> GSHMELTTTAARPGLRHRMQQLIYGFFTAQTLHVAVRLRIPDLLADGARDVGDLASATGADAPSLRRLLRALVFLEVLDEPAPGTFALTEQGEVLRADVTGSMRELVLLLSGPESWAAWGQLEHSVRTGEVAWEHVHGRSCFDHLMADPQRQAAFNAAMAEGSRAFVPTLLSAYDFGDLRTVVDVGGGSGALLAGVLAAHPHLRGTVFDTPDGVADAARTVAEQGVA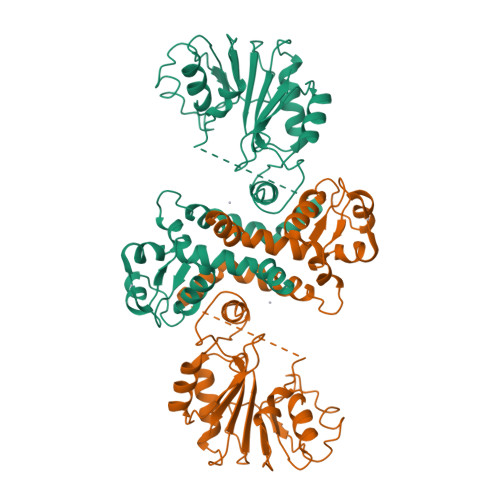DRCGVETGDFFVSVPPGADAYVLKSVLHDWDDEQCVEVLRTVRRAVRPDSRVILVESLMPTTVTTAPSVAQVVMNDLNMMVCHGGRERTVAEFRELLRVAGFRLESVTPCPAPSVVGILEAAPAPATGPDGS> SQAEFE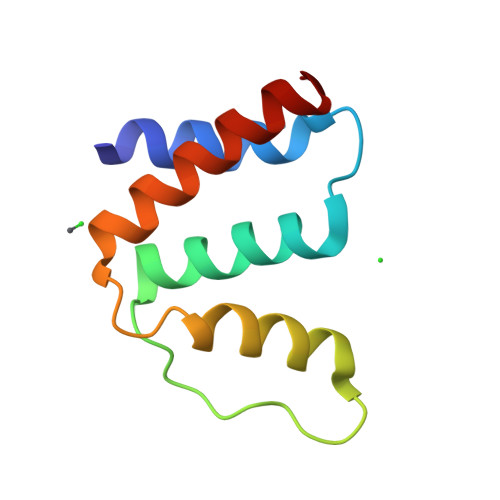KAAEEVRHLKTKPSDEEMLFIYGHYKQATVGDINTERPGMLDFTGKAKWDAWNELKGTSKEDAMKAYINKVEELKKKYGI>[6x]EVNGTI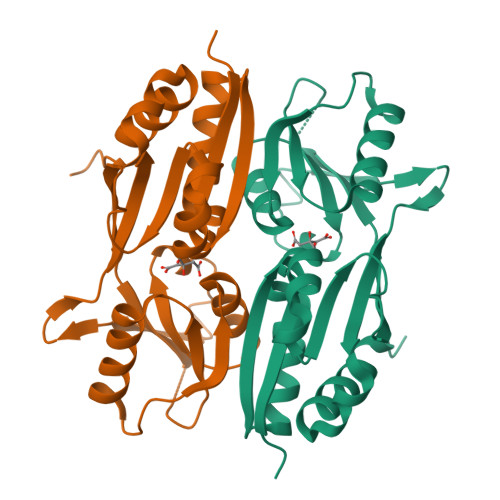SIGCSSLIGQTLLPEVLSLYNAQFPNVEIQVQVGSTEQIKANHRDYHVMITRGNKVMNLANTHLFNDDHYFIFPKNRRDDVTKLPFIEFQADPIYINQIKQWYNDNLEQDYHATITVDQVATCKEMLISGVGVTILPEIMMKNISKEQFEFEKVEIDNEPLIRSTFMSYDPSMLQLPQVDSFVNLMASFVEQPKA> VQSRTDVFNEQFANEALHPMTKVIFNGLDVNTEVQPLSDDFKQISDPKGYLTYSVKYEDQFTKKDKLRASEADDRIVGPTVNLFKYGAAVVNIDLNRDFFDTATGIDLTKGIPLVQDLLVPIGVTAGAEQSAEYVSGLLMVLFKVMTDNRLVIVGETTTPMSNTLSTVVNNVLRTTYHNNVGVNPALLRDFTQVNWLNRDITNMLQQAGTKYGLGLTETRLDYVRLVKTIVGHALNIDHFAASVLNINLRALMEANVTADDRIKALQ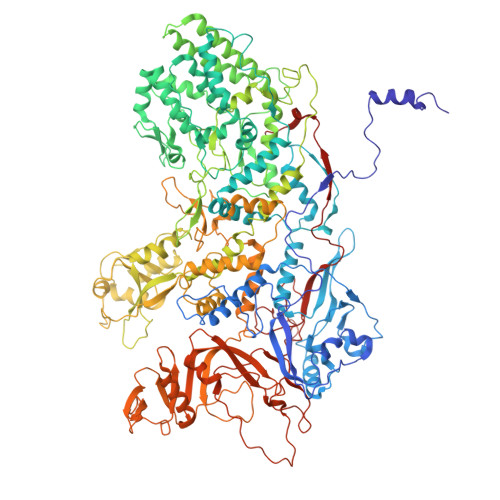AHSMISTQFHGPNQGALRPELAFDHDHIIRCLMLAAANYPRLEGIIVQINTGYVASANVIRPVSEKRYFPENLEQNQSAARLVSAVKARASEADISSIHLAIAREVSPMFNVHELKKIAESFEDPSSIVVVLEFILFALFFPTEFNRIKGDIQNVLLLFFSRWYPVEYGIFIQRGATYTINAAGEFEFSGRNEKWDQSLYLSEHFPALFSDVPLAGANTIIAIMRLFTPQGFLRTDDLAIAANFPRASRNPQTYIPYTNQRGTVTNEFASRFRTIVATLANVVNERAVQDDMQKATRSCTKQWLRHLETQFDNIAVAHTDHLSVVYATMSNFMLNFTNNFSGNHATFKPDQYVITSPEGSYKPIIERQGETVDGLTIIDTSIVWPILCQCTYPLVRQSGKGVDAVSIMEEIVYPDPSTTLSQSLSVAQVLSKLTLPDAFINMILSGGDSVVMRTYQTEADDDLDEGIRMTTYDQYLSHIRERLHITNVPDPIYITGASTPDQIAASVQATHVAVVLYQSGVINGSASTYLRENEVLVVMPDYYDVVSRFANANLQMNNNRYHESVLEIADIFDQADFIQTSDAVRQLRALMPTLSTSQIRHAIERIAQITDVDSTDYGKLTLRFLGTLTRSLKMQNAQIRRIRPDGTVLRYDDQIDIEAFRWSRYFLDELRLRRLSVGLRLITNPRIARRFDGVRIMYLTDDDPDPDFVPDVPEGYVAVQYAHRLFSSSLANKRNRVTYTHPPTGMAYPSPTGRPHVHMTINERAGMSKLVADNIIASVIKSNWVVDIHDIEYTAEVMTPSEGYTQHVDAESIMTAPKGKLFHLQFMDGLLRPEPSAFDPPASGEDMRLIYPLQPISVARSMRAIVNHNEVDRPRGAVAPSSYEMDTGTLSRNGDLLYSPVANGQVGIPKLEVDHISFSNVVSMMTANIRTGDDMAVERVNPDDVRAINIRNA>[2x]MSQNLFNVEDYRKLRQKRLPKMVYDYLEGGAEDEYGVKHNRDVFQQWRFKPKRLVDVS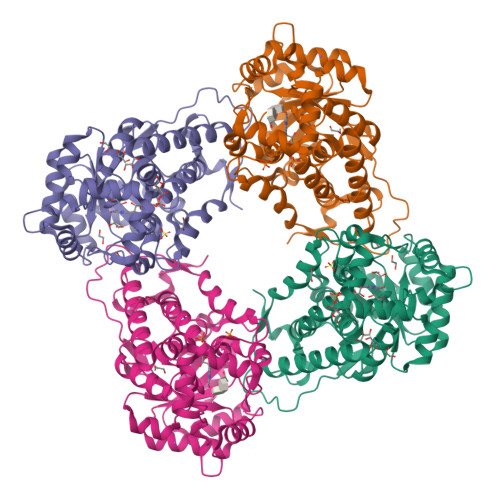RRSLQAEVLGKRQSMPLLIGPTGLNGALWPKGDLALARAATKAGIPFVLSTASNMSIEDLARQCDGDLWFQLYVIHREIAQGMVLKALHTGYTTLVLTTDVAVNGYRERDLHNRFKIPMSYSAKVVLDGCLHPRWSLDFVRHGMPQLANFVSSQTSSLEMQAALMSRQMDASFNWEALRWLRDLWPHKLLVKGLLSAEDADRCIAEGADGVILSNHGGRQLDCAISPMEVLAQSVAKTGKPVLIDSGFRRGSDIVKALALGAEAVLLGRATLYGLAARGETGVDEVLTLLKADIDRTLAQIGCPDITSLSPDYLQNEGVTNTAPVDHLIGKGTHAHHHHHH> MEGFIQNKRKKEKEGEEEEESKEKRKQINQLNKQKQEEEKIYQQKKDQKRKKYLYQRKEMTIFAETWEASEYQYRNKANLKTLPVNHLGKLAELKFDFVEYKAHQLIACHLYERMTIHCMNQYGLFKDFY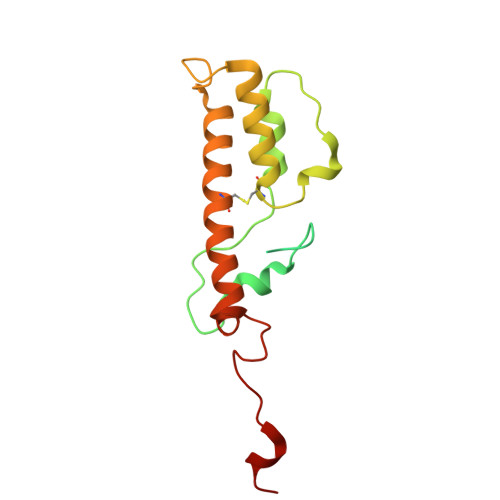RPECLDAQYYFKTCVELNAAYGIQKKFFPEHFVGSPYARPVPQFQQLGL methyl sulfate | C H4 O4 S 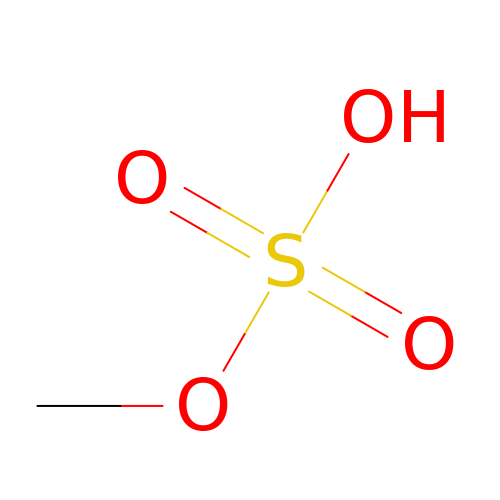| JZMJDSHXVKJFKW-UHFFFAOYSA-N> MGPVWRKHYITYRINNYTPDMNR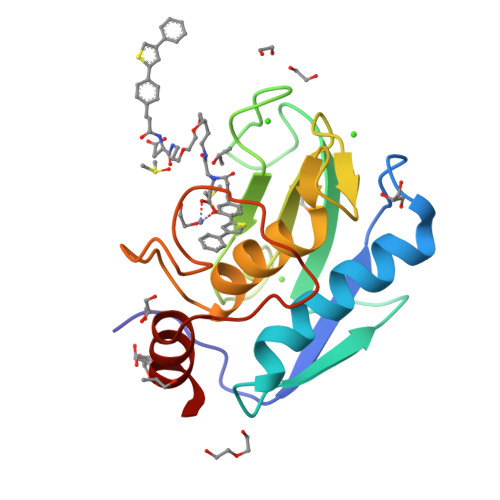EDVDYAIRKAFQVWSNVTPLKFSKINTGMADILVVFARGAHGDDHAFDGKGGILAHAFGPGSGIGGDAHFDEDEFWTTHSGGTNLFLTAVHAIGHSLGLGHSSDPKAVMFPTYKYVDINTFRLSADDIRGIQSLYG> MFPAAPSPRTPGTGSRRGPLAGLGPGSTPRTASRKGLPLGSAVSSPVLFSPVGRRSSLSSRGTPTRMFPHHSITESVNYDVKTFGSSLPVKVMEALTLAEVDDQLTINIDEGGWACLVCKEKLIIWKIALSPITKLSVCKELQLPPSDFHWSADLVALSYSSPSGEAHSTQAVAVMVATREGSIRYWPSLAGEDTYTEAFVDSGGDKTYSFLTAVQGGSFILSSSGSQLIRLIPESSGKIHQHILPQGQGMLSGIGRKVSSLFGILSPSSDLTLSSVLWDRERSSFYSLTSSNISKWELDDSSEKHAYSWDINRALKENITDAIWGSESNYEAIKEGVNIRYLDLKQNCDGLVILAAAWHSADNPCLIYYSLITIEDNGCQMSDAVTVEVTQYNPPFQSEDLILCQLTVPNFSNQTAYLYNESAVYVCSTGTGKFSLPQEKIVFNAQGDSVLGAGACGGVPIIFSRNSGLVSITSRENVSILAEDLEGSLASSVAGPNSESMIFETTTKNETIAQEDKIKLLKAAFLQYCRKDLGHAQMVVDELFSSHSDLDSDSELDRAVTQISVDLMDDYPASDPRWAESVPEEAPGFSNTSLIILHQLEDKMKAHSFLMDFIHQVGLFGRLGSFPVRGTPMATRLLLCEHAEKLSAAIVLKNHHSRLSDLVNTAILIALNKREYEIPSNLTPADVFFREVSQVDTICECLLEHEEQVLRDAPMDSIEWAEVVINVNNILKDMLQAASHYRQNRNSLYRREESLEKEPEYVPWTATSGPGGIRTVIIRQHEIVLKVAYPQADSNLRNIVTEQLVALIDCFLDGYVSQLKSVDKSSNRERYDNLEMEYLQKRSDLLSPLLSLGQYLWAASLAEKYCDFDILVQMCEQTDNQSRLQRYMTQFADQNFSDFLFRWYLEKGKRGKLLSQPISQHGQLANFLQAHEHLSWLHEINSQELEKAHATLLGLANMETRYFAKKKTLLGLSKLAALASDFSEDMLQEKIEEMAEQERFLLHQETLPEQLLAEKQLNLSAMPVLTAPQLIGLYICEENRRANEYDFKKALDLLEYIDEEEDININDLKLEILCKALQRDNWSSSDGKDDPIEVSKDSIFVKI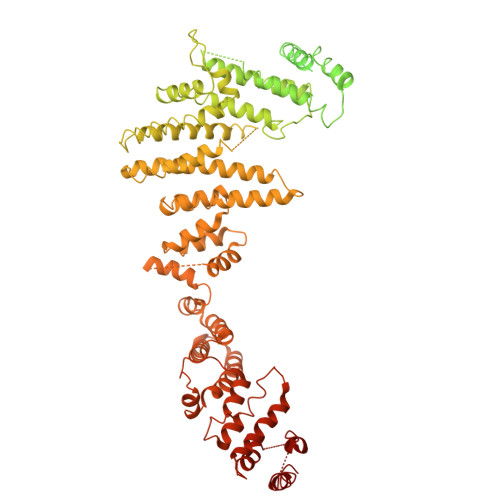LQKLLKDGIQLSEYLPEVKDLLQADQLGSLKSNPYFEFVLKANYEYYVQGQI> DYPAALQILMEGGTHMVCTGRTHTDRICRFKWLCYSNEAEEFIFFHGNTSVMLPNLGSRRFQPALLDLSTVEDHATQYFNFVELPAAALRFMPKPVFVPDVALIANRFNPDNLMHVFHDDLLPLFYTLRQFPGLAHEARLFFMEGWGEGAHFDLYKLLSPKQPLLRAQLKTLGRLLCFSHAFVGLSKITTWYQYGFVQPQGPKANILVSGNEIRQFARFMTEKLNASHTGVPLAEEYILVFSRTQNRLILNEAELLLALAQEFQMKTVTVSLEDHTFADVVRLVSNASMLVSMHGAQLVTTLFLPRGATVVELFPYAVNPDHYTPYKTLAMLPGMDLQYVAWRNMMPENTVTHPERPWDQGGITHLDRAQQAAILQSREVPRHLCCRNPEWLFRIYQDTKVDIPSLIQTIRRVVAAPGPAKQKAAAGLYPGKVREARCQASVHGASEARLTVSWQIPWNLKYLKVAEVKYEVWLQEQGEAAYVPYILALQNHTFTENIKPFTTYL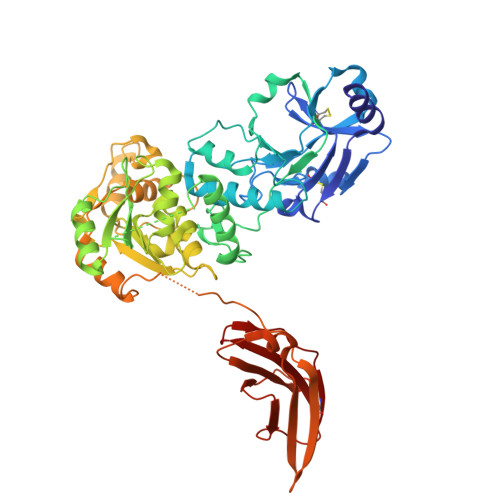VWVRCIFNKILLGPFADVLVCNT>[6x]MSKSVFVGELTWKEYEARVAAGDCVLMLPVGALEQHGHHMCMNVDVLLPTAVCKRVA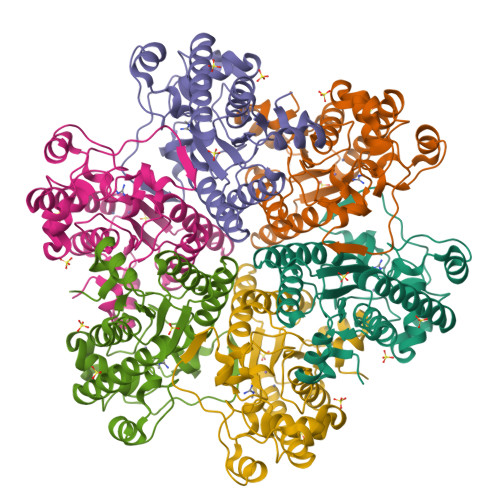ERIGALVMPGLQYGYKSQQKSGGGNHFPGTTSLDGATLTGTVQDIIRELARHGARRLVLMNGHYENSMFIVEGIDLALRELRYAGIQDFKVVVLSYWDFVKDPAVIQQLYPEGFLGWDIEHGGVFETSLMLALYPDLVDLDRVVDHPPATFPPYDVFPVDPARTPAPGTLSSAKTASREKGELILEVCVQGIADAIREEFPPT>MMKIVPPKPFFFEAGERAVLLLHGFTGNSADVRMLGRFLESKGYTCHAPIYKGHGVPPEELVHTGPDDWWQDVMNGYQFLKNKGYEKIAVAGLSLGGVFSLKLGYTVPIEGIVTMCAPMYIKSEETMYEGVLEYAREYKKREGKSEEQIEQEME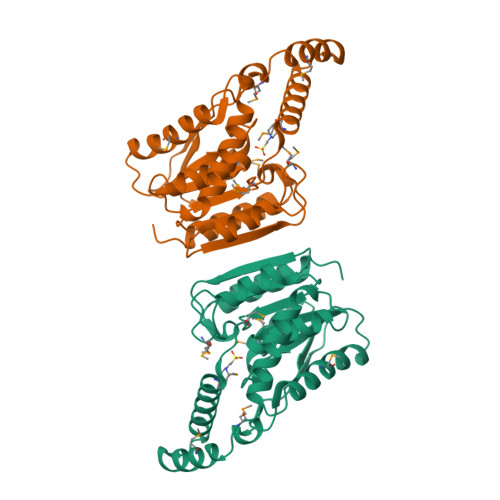RFKQTPMKTLKALQELIADVRAHLDLVYAPTFVVQARHDEMINPDSANIIYNEIESPVKQIKWYEQSGHVITLDQEKDQLHEDIYAFLESLDW[2x]The lpgD gene was identified by a targeted mutant screen, and the purified protein exhibited cation-dependent phosphodiesterase activity converting LPG to a cyclic-lysophosphatidic acid (cLPA) intermediate that is hydrolyzed to lysophosphatidic acid (LPA). The 2.1 Å crystal structure shows LpgD adopts the canonical glycerophosphodiester phosphodiesterase (GDPD) TIM barrel fold except for the positioning and length of helix α6 and sheet β7 that create a hydrophobic docking platform for the LPG acyl chain. The specific physiological function of LpgD in S. aureus is to re-cycle LPG into the PG biosynthetic pathway at the LPA acyltransferase step to maintain membrane PG molecular species homeostasis.

We postulated that the actual ligand associated with His93 would most logically be a water molecule and that P2 was partially displacing the water due to the low pH and high phosphate concentration in the crystallization condition. The refined 2.4 Å structure showed a single dihydrogen phosphate ion (P1) located in the same position in the active site as was present in the initial, lower pH structure. However, the low occupancy phosphate (P2) is clearly replaced by a water molecule hydrogen bonded to His93 as illustrated by the Fo-Fc simulated annealing omit map. These data suggest His93 is hydrogen bonded to a water molecule in substrate-free LpgDΔN. The LpgDΔN structure lacks a divalent cation; however, Mn2+ is proposed to bind to the same three acidic residues as the Ca2+ of BsGlpQ. The release of glycerol allows water to enter the active site and His93 acts as general base that catalyzes the water addition to the cLPA intermediate to form the LpgD-LPA product complex.

> MAINKNKVITKKQTIPAFFKGNAPYIFAHRGGMALRPEQTQLAFDYAKQLGVDGFETDVRLTKDQQLIVFHDATVDRTTNGSGKVSAHTLAELKKLDAAYHFKDINGLTPYRGHAHTAILTFDELLKQYPDMYINVDLKDAPESYEGSIAPQIMFDTIAENQAFDRVLVTSFYKEQIVRFNKIAQGSVAIGASQQEVTEAFLKYHLLGGRYYQPLAQTFQMPTHFKGIDLTSSRFIKWLNDMNIIPGYYGVNSINLMNDLYQKGAHTIVTDRPDLAQQFKQTIPNKLEHHHHHH Here, we present a new pipeline, SIMBAD (Sequence-Independent Molecular replacement Based on Available Databases), which can be used for both contaminant and brute-force approaches. In this section, we present three cases in which SIMBAD has been used to determine a difficult-to-solve case owing to the unwitting crystallization of a contaminant. All cases involve the crystallization of a known contaminant. Although the targets were ultimately of low importance for the structural insights that they provided, their solution prevented further misdirected effort on the part of the researchers involved.

Protein A was produced in E. coli TOP10F′ cells, overexpressed as a recombinant fusion with a 6×His tag and purified by successive metal-affinity and size-exclusion chromatography steps. Mass spectrometry (4800 MALDI-TOF/TOF, Abi Sciex) confirmed the anticipated identity of the purified target protein. Crystals were thereafter obtained by vapour diffusion after three months of incubation at 19°C in 600 nl drops composed of a 1:1 mixture of protein and reservoir solutions in a sitting-drop setup with 90 µl reservoir solution [0.085 M Na HEPES pH 7.5, 17%(w/v) PEG 4000, 15%(v/v) glycerol, 8.5%(v/v) 2-propanol or 0.1 M HEPES pH 7.0, 20%(w/v) PEG 6000, 1.0 M lithium chloride] in the reservoir. The crystals grew in space group P1, with unit-cell parameters a = 69.34, b = 90.14, c = 114.76 Å, α = 107.10, β = 105.60, γ = 95.98°, and diffracted X-rays to 2.93 Å resolution. Initial phasing attempts failed using molecular replacement (MR) with models displaying 20–30% sequence identity to our target (the best hits available in the PDB) as search probes. Ab initio/MR phasing strategies such as ARCIMBOLDO also proved to be unsuccessful, likely owing to limited resolution. We decided to optimize the crystallization conditions with the aim of obtaining crystals that diffracted X-rays to higher resolution, as well as to apply experimental phasing methods. Similar crystals did grow in the optimization plates after three-month incubations from 2 µl hanging drops with 1 ml reservoir solution in the reservoir, indicating that crystallogenesis was reproducible, even though new protein batches were used. Mass spectrometry with a Quadrupole-Orbitrap hybrid mass spectrometer (Q-Exactive Plus, Thermo) revealed that the E. coli catalase HPII was present in an ∼1:40 ratio relative to our target in the protein samples employed for crystallization. Even though catalase HPII is a known contaminant that is prone to crystallize, the P1 crystal lattice had not previously been reported, escaping a PDB-wide search as demonstrated by the SIMBAD lattice-parameter search.

>[4x]MSQHNEKNPHQHQSPLHDSSEAKPGMDSLAPEDGSHRPAAEPTPPGAQPTAPGSLKAPDTRNEKLNSLEDVRKGSENYALTTNQGVRIADDQNSLRAGSRGPTLLEDFILREKITHFDHERIPERIVHARGSAAHGYFQPYKSLSDITKADFLSDPNKITPVFVRFSTVQGGAGSADTVRDIRGFATKFYTEEGIFDLVGNNTPIFFIQDAHKFPDFVHAVKPEPHWAIPQGQSAHDTFWDYVSLQPETLHNVMWAMSDRGIPRSYRTMEGFGIHTFRLINAEGKATFVRFHWKPLAGKASLVWDEAQKLTGRDPDFHRRELWEAIEAGDFPEYELGFQLIPEEDEFKFDFDLLDPTKLIPEELVPVQRVGKMVLNRNPDNFFAENEQAAFHPGHIVPGLDFTNDPLLQGRLFSYTDTQISRLGGPNFHEIPINRPTCPYHNFQRDGMHRMGIDTNPANYEPNSINDNWPRETPPGPKRGGFESYQERVEGNKVRERSPSFGEYYSHPRLFWLSQTPFEQRHIVDGFSFELSKVVRPYIRERVVDQLAHIDLTLAQAVAKNLGIELTDDQLNITPPPDVNGLKKDPSLSLYAIPDGDVKGRVVAILLNDEVRSADLLAILKALKAKGVHAKLLYSRMGEVTADDGTVLPIAATFAGAPSLTVDAVIVPCGNIADIADNGDANYYLMEAYKHLKPIALAGDARKFKATIKIADQGEEGIVEADSADGSFMDELLTLMAAHRVWSRIPKIDKIPA>[3x]MPDFLGHAENPLREEEWARLNETVIQVARRSLVGRRILDIYGPLGAGVQTVPYDEFQGVSPGAVDIVGEQETAMVFTDARKFKTIPIIYKDFLLHWRDIEAARTHNMPLDVSAAAGAAALCAQQEDELIFYGDARLGYEGLMTANGRLTVPLGDWTSPGGGFQAIVEATRKLNEQGHFGPYAVVLSPRLYSQLHRIYEKTGVLEIETIRQLASDGVYQSNRLRGESGVVVSTGRENMDLAVSMDMVA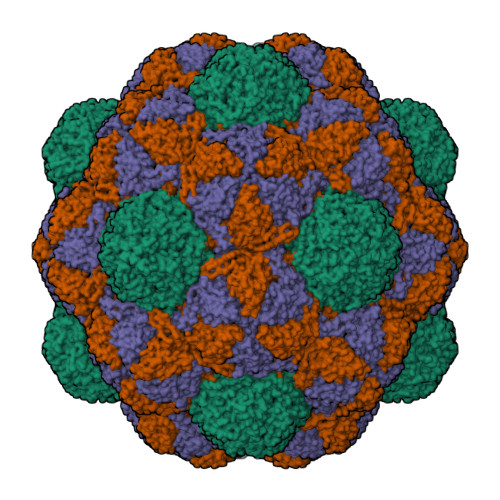AYLGASRMNHPFRVLEALLLRIKHPDAICTLEGAGATERR> GSHMELTPDQQTLLHFIMDSYNKQRMPQEITNKILKEAFSAEENFLILTEMATNHVQVLVEFTKKLPGF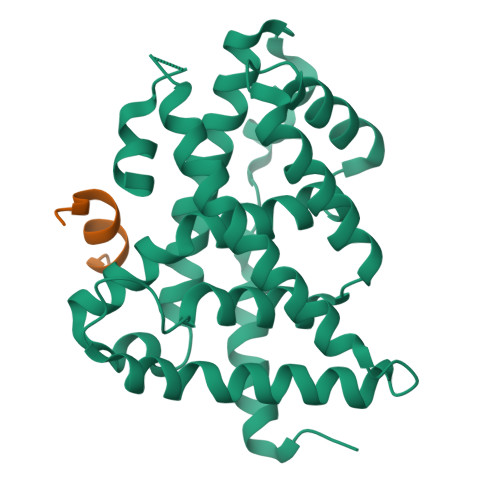QTLDHEDQIALLKGSAVEAMFLRSAEIFNKKLPSGHSDLLEARIRNSGISDEYITPMFSFYKSIGELKMTQEEYALLTAIVILSPDRQYIKDREAVEKLQEPLLDVLQKLCKIHQPENPQHFACLLGRLTELRTFNHHHAEMLMSWRVNDHKFTPLLCEIWDVQ;> KDHQLLRYLLDKDE> MSGNREQVFPTRMTLGLMKTKLKGANQGYSLLKRKSEALTKRFRDITKRIDDAKQKMGRVMQTAAFSLAEVSYATGENIGYQVQESVSTARFKVRARQENVSGVYLSQFESYIDPEINDFRLTGLGRGGQQVQRAKEIYSRA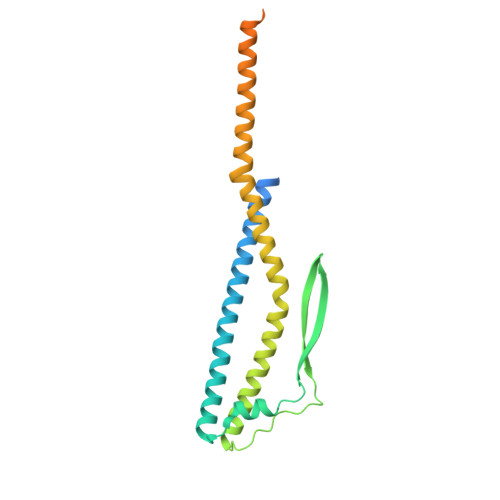VETLVELASLQTAFIILDEVIKVTNRRVNAIEHVIIPRTENTIAYINSELDELDREEFYRLKKVQEKKQNETAKLDAEMKLKRDRAEQDASEVAADEEPQGETLVADQEDDVIF>[2x]MSAHRTLLLRLSDSGEPVTSCSYGQGVLTLPSLPLPQGKKLGDMPVYTVKLAIPAGSPVTRDGLIWTNCPPDFSTQFDREKFYKKIIKTSFHEDDHIDLDIYVPGTYCFYLSFKNDKDELETTRKFYFVVLPILSVNDKFIPLNSIAMQSVVSKWMGPTIKDWEKVFARVASKKYNMIHFTPLQHRGESNSPYSIYDQLEFDPTVFKSEKEVADMVERLRTEHNILSLTDIVFNHTANNSQWLLDHPEAGYNHKTSPHLISAIELDKKLLDFSEQMEALGYPVDLKTVDDLIKVMDGIKEHVIGELKLWEFYVVDVKQTVSELREKWGNSKSWSDDNIPSKDDSTNLAQFVRDNATEPGFGSLGERGSNKINIDKFAAILKKLHSEDYNNGIEELATKILNDINLPFYKEYDDDINEVLEQLFNRIKYLRIDDHGPKQGPITKKLPLSEPYFTRFKAKDGEEYALANNGWIWDGNPLVDFASSQSKAYLRREVIVWGDCVKLRYGKGPSDSPYLWERMSKYVEMNARIFNGFRINNCHSTPLHVGQYFLDVARRVNPNLYVVAELFSGSEAMDCLFVERLGISSLIREAMQAWSEEELSRLVHRHGGRPIGSYKFVPLDDFPYPADVKIDEEYCAYNPDDHSVKCVSEIMIPKTLTATPPHALFMDCTHDNETPNQKRTVEDTLPNAALVAFCSSAIGSVYGYDEVFPQLLDLVQEKRTYSCAENTGISKVKTLLNNMREEIASEAVDIEDSEMHVHHDGQYITFHRTNAKNGKGWYLVARTKFHSSGDQMLPRIKLSQTKATFKAAFSLERTGDAPISDEIIEGIPTKLRELTGFDIGFDENTKETSILLPQDFPQGSIVIFETQQLGIDDSLDHFIRSGAIKATEKLSLESINYVLYRAEQEEYDYSEGRSGAYDIPDYGK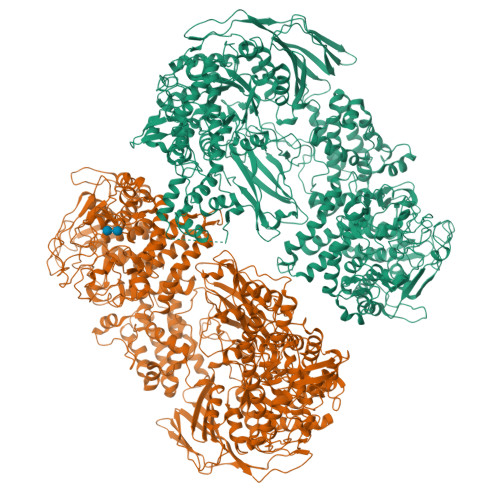PVYCGLQGWVSILRKIIFYNDLAHPLSNNLRNGHWAVDYVVNRLDLYKDKEGVAEVQEWLRSRMERIKQLPSYLVPSFFALVVGIMYGCCRLRAMQLMSDNVGKSTVFVQSLAMTSIQMVSAMKSTSILPDQNIAAMAAGLPHFSTNYMRCWGRDVFISLRGLLLTTGRYEEAKEHILAFAKTLKHGLIPNLLDAGRNPRYNARDAAWFFVQAIQDYVTIVPGGVSLLQEKVTRRFPLDDEYIPYDDPKAFSYSSTIEEIIYEILNRHAGGIKYREANAGPNLDRVMKDEGFNVEVNVDWETGLIHGGSQFNCGTWMDKMGESEKANSVGVPGTPRDGAAVEINGLLKSCLRFVLQLSKDGKFKYTEVTKPDGSKISLSSWNDLLQENFERCFYVPKNKEDDNKFEIDATIINRRGIYKDLYRSGKPYEDYQFRPNFTIAMVVAPELFTPDYAAGAIELADQVLRGPVGMRTLDPSDYNYRPYYNNGEDSDDFATSKGRNYHQGPEWVWCYGYFIRAYHYFNFLTNPKCQVEGSAKKLKPSSYLYRKLYSRLLKHREWIENSPWAGLAELTNKDGEVCNDSSPTQAWSTGCLLDLFYDLWISYEELEHHHHHH> PLKVEKFATANRGNGLRAVTPLRPGELLFRSDPLAYTVCKGSRGVVCDRCLLGKEKLMRCSQCRVAKYCSAKCQKKAWPDHKRECKCLKSCKPRYPPDSVRLLGRVVFKLMDGAPSESEKLYSFYDLESNINKLTEDRKEGLRQLVMTFQHFMREEIQDASQLPPAFDLFEAFAKVICNSFTICNAEMQEVGVGLYPSISLLNHSCDPNCSIVFNGPHLLLRAVRDIEVGEELTICYLDMLMTSEERRKQLRDQYCFECDCFRCQTQDKDAD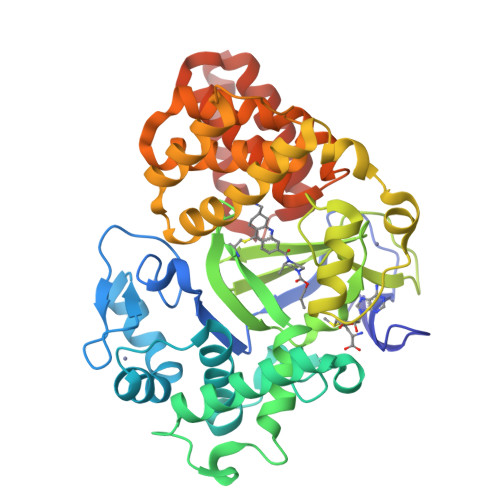MLTGDEQVWKEVQESLKKIEELKAHWKWEQVLAMCQAIISSNSERLPDINIYQLKVLDCAMDACINLGLLEEALFYGTRTMEPYRIFFPGSHPVRGVQVMKVGKLQLHQGMFPQAMKNLRLAFDIMRVTHGREHSLIEDLILLLEECDANI> MADPRTDNRNRKIPDAQVDAIKVPPHSLEAEQSVIGGLLLDNERWDTVSEHVMTQDFYSRPHRLIFDGVKSILEAGKPLDLITLSEYLEQREQLEDVGGFAYLADLAKNTPSAANINAYAEIVAERALVRNLIGVA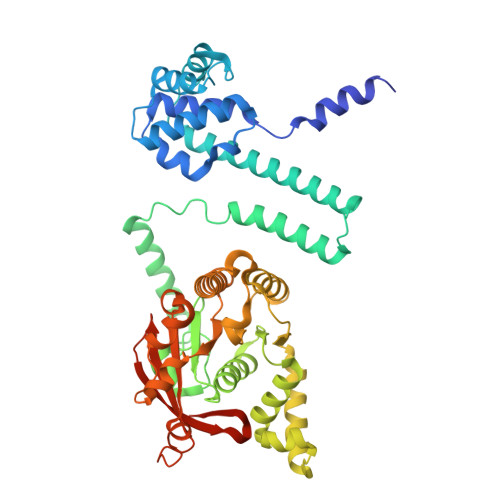NEIADAGYDPQGRNAEDLLDLAESKVFAIAEARTSENEGPKNVDSILERTLERIELLYKTPQDGVTGVNTGFTDLNKKTAGLQGSDLIIVAARPSMGKTTFAMNLCENAAMEQDKPVLIFSLEMPAEQIMMRMLASLSRVDQTKIRTGQLDDEDWARISSTMGILMEKKNMYIDDSSGLTPTEVRSRARRIAREHGGLSLIMVDYLQLMRVPALTDNRTLEIAEISRSLKALAKELNVPVVALSQLNRSLEQRADKRPVNSDLRESGSIEQDADLIMFIYRDEVYHPDSPLKGTAEIIIGKQRNGPIGSVRLTFQGHYSRFDNYAGPAFDDEHHHHHH>[4x]MVLETLKQGLDSSQIHEALIQLDSYPREPVDLDASMVLIKFVIPVYPSLPERSKVILRRLASKSFTFLCQIVTFSRTISGRDGLQEIRIYQEILEDIISFEPGCLTFYLKASTTSKADRDSIKALFFGSKLFNVLANRIDMAKYLGYLRLQWKFLLESNETDPPGFLGEWLVSSFLLNPVLAADMLLGELFLLKESYFFSFQKIISASSLIDQKRLIAKFLLPYIQVIVTLENLNDVRKILRRFDLDKIISLSVLFEIQSLPLK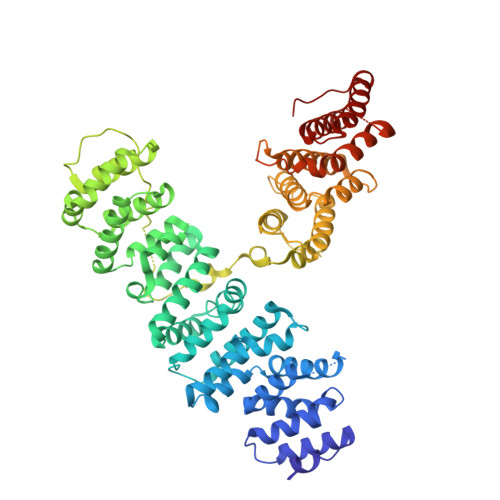EVIVRLMSNHSSTKFVSALVSKFADFTDEEVDTKTCELLVLFAVHNLNHSQREEIAHDERFLNGVTKHLGSNEREARERAMFIAKLLSGGHLKYESDFKINIPNVKFESNSDDKIIDFQSLKREIVKRIVFLKDLMKEYEKTGESRKAPLIPLLKQTVKLIRQKADFQLEVGYYAQGILSSIVCLNNEFDEPLFEQWRINALTSILVVLPEKVNGAINILFNSELSLQQRMSLLSALGLSARELRGLDDPTIVKPKFDFPTNRLPWDDQSHHNSRLVEVQESTSMIKKTKTVWKSRKLGKDREKGTQNRFRKYAGLFFYPLAHGWLNGIDVGTYNQLFKSHYLTTLRIIYSCANPVHDFESMTELMNHIISSAIEEGISLNKG> KELNDLEKKYNAHIGVYALDTKSGKEVKFNSDKRFAYASTSKAINSAILLEQVPYNKLNKKVHINKDDIVAYSPILEKYVGKDITLKALIEASMTYSDNT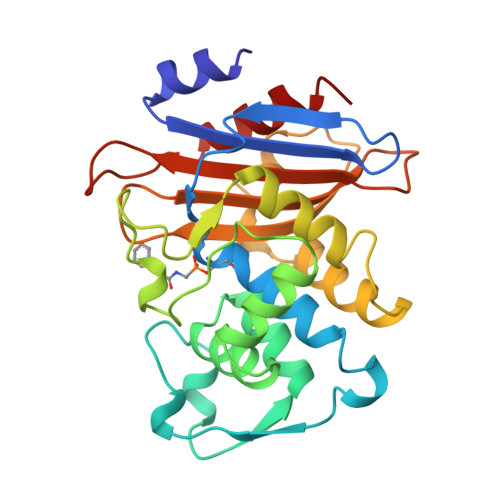ANNKIIKEIGGIKKVKQRLKELGDKVTNPVRYEIELNYYSPKSKKDTSTPAAFGKTLNKLIANGKLSKENKKFLLDLMLNNKSGDTLIKDGVPKDYKVADKSGQAITYASRNDVAFVYPKGQSEPIVLVIFTNKDNKSDKPNDKLISETAKSVMKEF> GG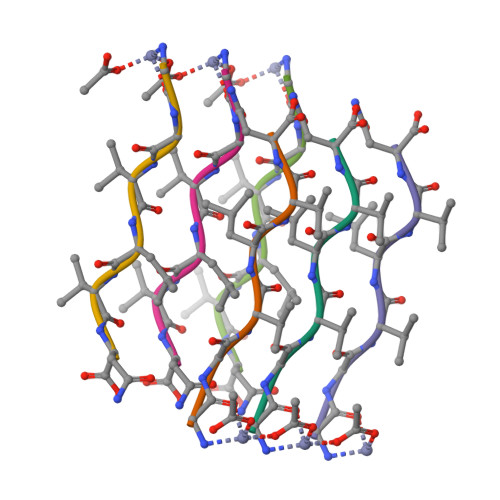VLVN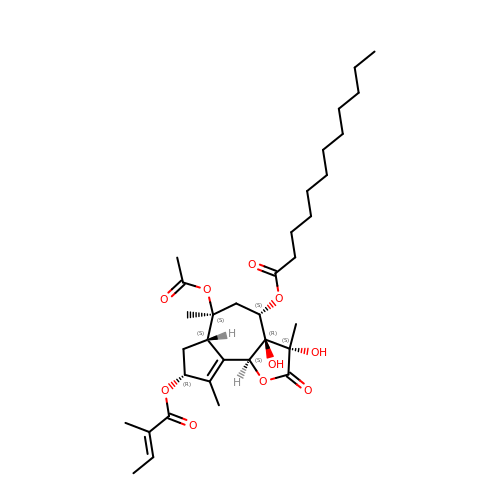(3S,3aR,4S,6S,6aS,8R,9bS)-6-(acetyloxy)-3,3a-dihydroxy-3,6,9-trimethyl-8-{[(2Z)-2-methylbut-2-enoyl]oxy}-2-oxo-2,3,3a,4,5,6,6a,7,8,9b-decahydroazuleno[4,5-b]furan-4-yl dodecanoate | C34 H52 O10 | PTOLDSROGFHZGU-VFCZBPRFSA-N>SNPYSYAMSTEEARFLTYHMWPLTFLSPSELARAGFYYIGPGDRVACFACGGKLSNWEPKDDAMSEHRRHFPNC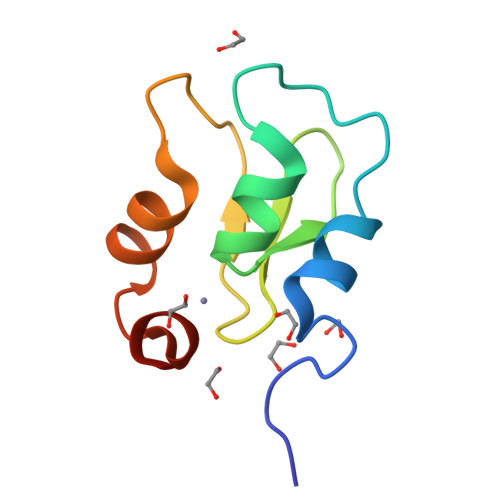PFLENSLET[2x]>[2x]GGADQKGPVFLKEPTNRIDFSNSTGAEIECKASGNPMPEIIWIRSDGTAVGDVPGLRQISSDGKLVFPPFRAEDYRQEVHAQVYACLARNQFGSIISRDVHVRAVVIQSYESEADNEYVIRGNSVVMKCEIPSYVADFVFVDLWLDSEGRNYYPNNAA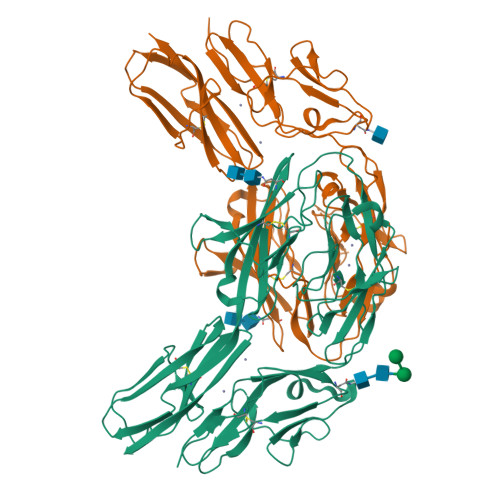ETDGKYLVLPSGELHIREVGPEDGYKSYQCRTKHRLTGETRLSATKGRLVITEPVGSKAPTFATASKISSLLGSSSSDIVLLCQAQAFPVPYTRWYKFIEGTTRKQAVVLNDRVKQVSGTLIIKDAVVEDSGKYLCVVNNSVGGESVETVLTVTAPLSAKIDPPTQTVDFGRPAVFTCQYTGNPIKTVSWMKDGKAIGHSEPVLRIESVKKEDKGMYQCFVRNDQESAEASAELKLGG>[12x]XGEIGQALKEIGKALKEIGY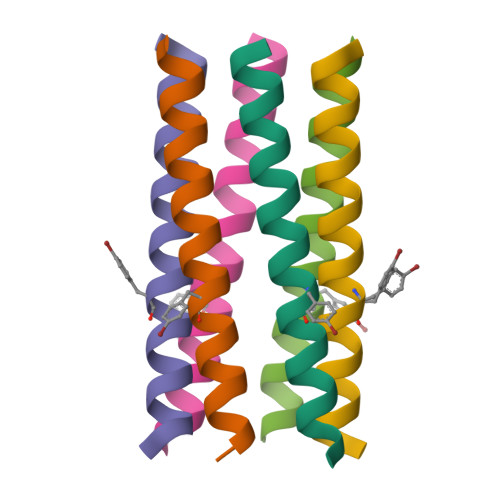ALKEIGQALKGX[(5-phenylpyridin-2-yl)methyl]phosphonic acid | C12 H12 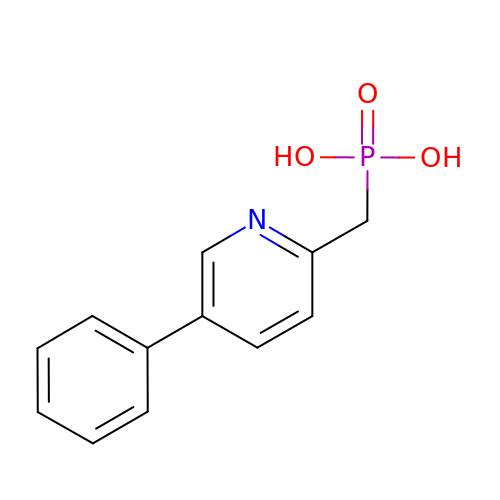N O3 P | JTYLHYFDHHMHKD-UHFFFAOYSA-N>[6x]MERLRQIASQATAASAAPARPAHPLDPLSTAEIKAATNTVKSYFAGKKISFNTVTLREPARKAYIQWKEQGGPLPPRLAYYVILEAGKPGVKEGLVDLASLSVIETRALETVQPILTVEDLCSTEEVIRNDPAVIEQCVLSGIPANEMHKVYCDPWTIGYDERWGTGKRLQQALVYYRSDEDDSQYSHPLDFCPIVDTEEKKVIFIDIPNRRRKVSKHKHANFYPKHMIEKVGAMRPEAPPINVTQPEGVSFKMTGNVMEWSNFKFHIGFNYREGIVLSDVSYNDHGNVRPIFHRISLSEMIVPAGSPEFPHQRKHALDIGEYGAGYMTNPLSLGCDCKGVIHYLDAHFSDRAGDPITVKNAVCIHEEDDGLLFKHSDFRDNFATSLVTRATKLVVSQIFTAANYEYCLYWVFMQDGAIRLDIRLTGILNTYILGDDEEAGPWGTRVYPNVNAHNHQHLFSLRIDPRIDGDGNSAAACDAKSSPYPLGSPENMYG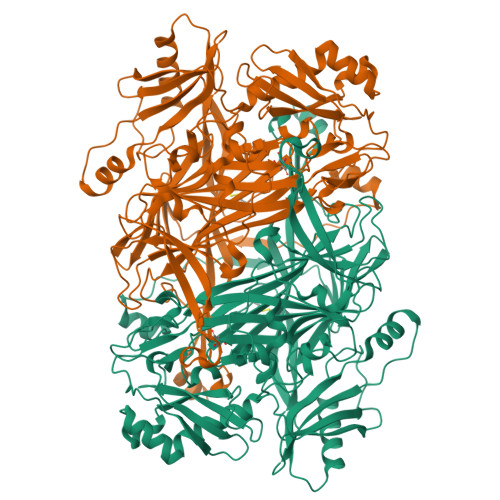NAFYSEKTTFKTVKDSLTNYESATGRSWDIFNPNKVNPYSGKPPSYKLVSTQCPPLLAKEGSLVAKRAPWASHSVNVVPYKDNRLYPSGDHVPQWSGDGVRGMREWIGDGSENIDNTDILFFHTFGITHFPAPEDFPLMPAEPITLMLRPRHFFTENPGLDIQPSYAMTTSEAKRAVHKETKDKTSRLAFEGSCCGK> MLIGDFSKGYLFHTVAGKHQDLKYISPEIMASVLNGKFANLIKEFVIIDCRYPYEYEGGHIKGAVNLHMEE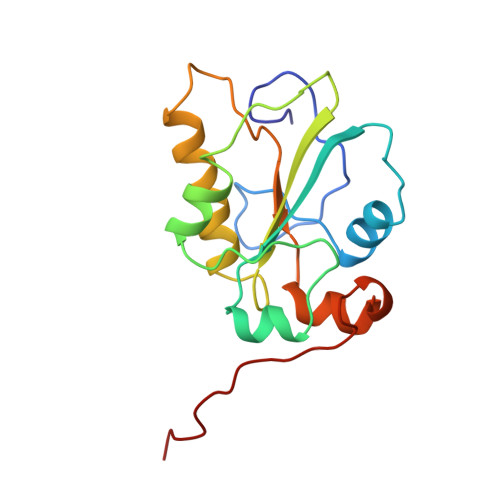EVEDFLLKKPIVPTDGKRVIVVFHCEFSSERGPRMCRYVRERDRLGNEYPKLHYPELYVLKGGYKEFFMKCQSYCEPPSYRPMHHEDFKE>[3x]SDNNSEDEMLMVMPNASTSSGESGRCFDDERIKIVPHIGWRAGIGDRDFDIELDENIANWFEGFRDSFKTFKKGPLISQRLQMFYMNTRNPYEWSLKLFANCPDHNSPKSNSLAYTVLEEMRNFKKHYNLGTDQLVDDNLRMVAFNFVAKQGHCLLFRMVVDIFEFLQCRDLFIPKVREMIARKQYKEAGQIAIDLELFEEFDEHDFVMPLFMQDKISIAEDYLNKAERLQGPVVQLLDSFFDKR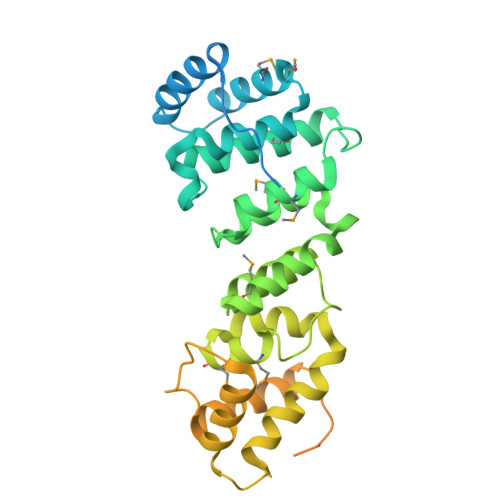QSVESHCSRYITEHEVTDVYYSKLHQKPLSKLVQRLAKNYNIPRQFTPNVNKMKNFGALQFLVHKRYYEKSLNKDSWDEMVRDTVSETDRELQLELVCLCSNFNDQPEAAKWAFHYQLKRSDLPLLVQDYILEQEG>MGIQGLAKLIADVAPSAIRENDIKSYFGRKVAIDASMSIYQFLIAVRQGGDVLQNEEGETTSHLMGMFYRTIRMMENGIKPVYVFDGKPPQLKSGELAKRSERRAEAEKQLQQAQAAGAEQEVEKFTKRLVKVTKQHNDECKHLLSLMGIPYLDAPSEAEASCAALVKAGKVYAAATEDMDCLTFGSPVLMRHLTASEAKKLPIQEFHLSRILQELGLNQEQFVDLCILLGSDYCESIRGIGPKRAVDLIQKHKSI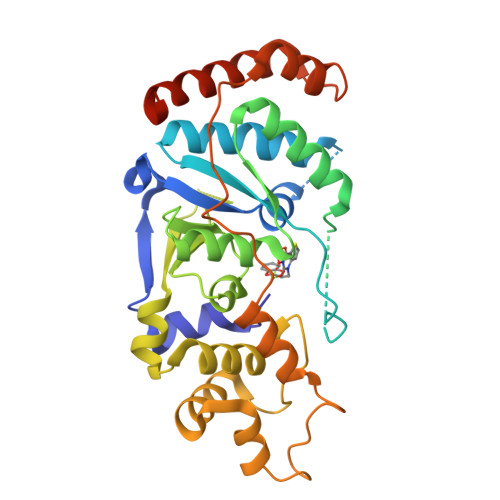EEIVRRLDPNKYPVPENWLHKEAHQLFLEPEVLDPESVELKWSEPNEEELIKFMCGEKQFSEERIRSGVKRLSKSRQGSTLEVLFQGPGGGHHHHHH[2x]>[2x]MTPSHP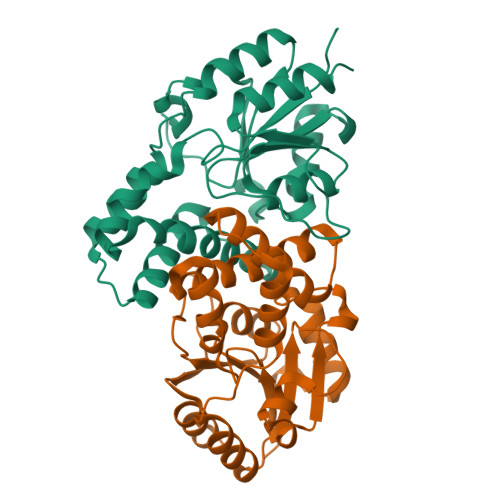ARPSRSGILVFDVNETLLDLTSLSPLFERVFGDAKVLREWFPELILYSQTLTLTGLYRPFGEIAAAVFEMVAANHQAKVTPDDIAELKTRLTSMPAYPDVAPALTRLQDAGFRLVTLTNSAPSPAPSPLEKAGIASFFEAHLTVHSSQRFKPHPSVYDSTAETLGAKPEELCMIACHIWDTIGAQARGWRGGFVARPHNTPLTLAEVPQPDFIGRDMGELADQLIASLTA>GPLGSVPPTIEQKTRAFTVPNIPLQTLSNSRFPSLIQGMILSPDASQVVQFQNGRCLIDGQLLGTTPATSGQLFRVRGKINQGARTLNLTEVDGKPFMAFDSPAPVGFPDFGKCDWHMRISKTPNNTSSGDPMRSVSVQTNVQGFVPHLGSIQFDEVFNHPTGDYIGTIEWISQPSTPPGTDINLWEIPDYGSSLSQAANLAPPVFPPGFGEALVYFVSAFPG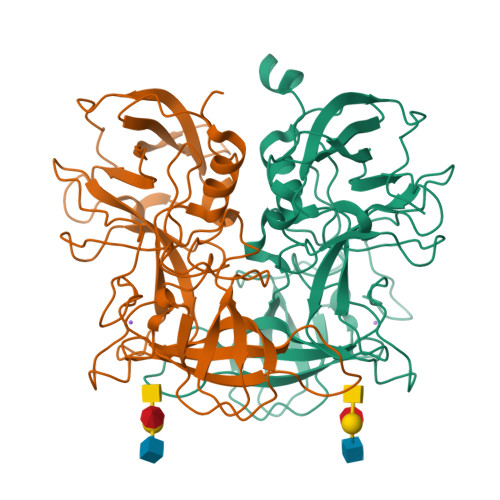PNNRSAPNDVPCLLPQEYITHFVSEQAPTMGDAALLHYVDPDTNRNLGEFKLYPGGYLTCVPNGVGAGPQQLPLNGVFLFVSWVSRFYQLKPVGTASTARSRL[2x]>[3x]MKHLTTMSELSTEEIKDLLQTAQELKSGKTDNQLTGKFAANLFFEPSTRTRFSFEVAEKKLGMNVLNLDGTSTSVQKGETLYDTIRTLESIGVDVCVIRHSEDEYYEELVSQVNIPILNAGDGCGQHPTQSLLDLMTIYEEFNTFKGLTVSIHGDIKHSRVARSNAEVLTRLGARVLFSGPSEWQDEENTFGTYVSMDEAVESSDVVMLLRIQNERHQSAVSQEGYLNKYGLTVERAERMKRHAIIMHPA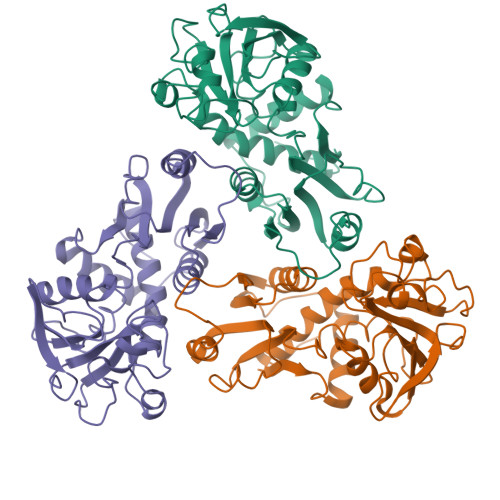PVNRGVEIDDSLVESEKSRIFKQMKNGVFIRMAVIQCALQTNVKRGEAAY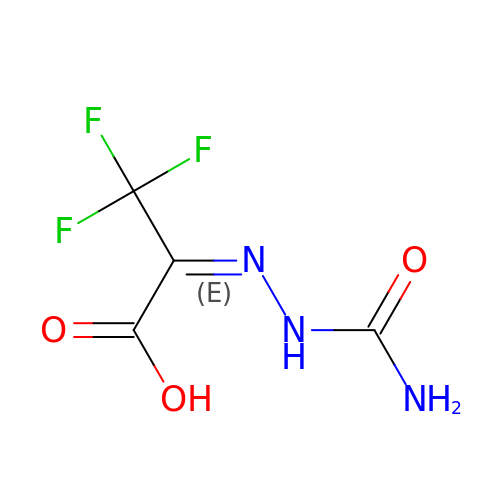(2E)-2-(2-carbamoylhydrazinylidene)-3,3,3-trifluoropropanoic acid | C4 H4 F3 N3 O3 | FPZRQHLDHOFSAY-XLUWADSXSA-N> GMTARNILSYSYEEYVEKITAFHGYPAPGVLIGGFMVDLAVKNLPEGILYDAICETRTCLPDAVQLLTPCTFGNGWLTVLPMGLFAVSLYDKFTGEGVRVFLDVEKMGPWQEIRNWFLKLKTKKEQDSERLFK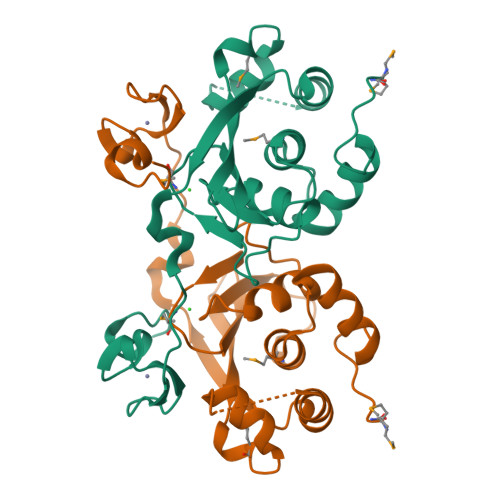EIREAGPDILELRNVKLKPGFLEKKHKGKIVLCPQCREAYPAQDGELCLSCQGGSPYL>[6x]AEIGGDHGYNATNIAAGQTSGAVTQIGPAVMGMVRRAIPNLIAFDICGVQPMNSPTGQVFALRAVYGKDPVAAGAKEAFHPMYGPDAMFSGQGAAKKFPALAASTQTTVGDIYTHFFQETGTVYLQASVQVTIDAGATDAAKLDAEIKKQMEAGALVEIAEGMATSIAELQEGFNGSTDNPWNEMGFRIDKQVIEAKSRQLKAAYSIELTQDLRAVHGMDADAELSGILATEIMLEINREVVDWINYSAQVGKSGMTLTPGSKAGVFDFQDPIDIRGARWAGESFKALLFQIDKEAVEIARQTGRGEGNFIIASRNVVNVLASVDTGISYAAQGLATGFSTDTTKSVFAGVLGGKYRVYIDQYAKQDYFTVGYKGPNEMDAGIYYAPYVALTPLRGSDPKNFQPVMGFKTRYGIGINPFAESAAQAPASRIQSGMPSILNSLGKNAYFRRVYVKGI;>MTFTVDITPKTPTGVIDETKQFTATPSGQ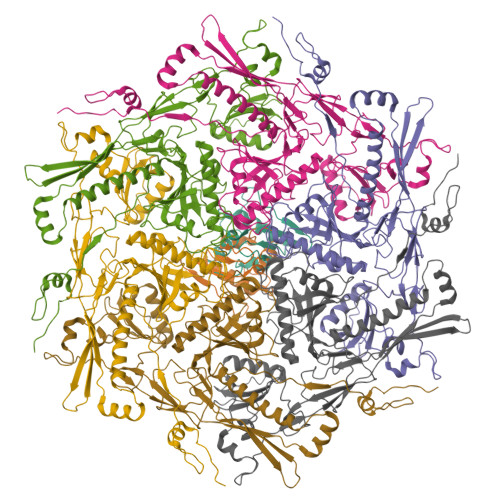TGGGTITYAWSVDNVPQDGAEATFSYVLKGPAGQKTIKVVATNTLSEGGPETAEATTTITVKNKTQTTTLAVTPASPAAGVIGTPVQFTAALASQPDGASATYQWYVDDSQVGGETNSTFSYTPTTSGVKRIKCVAQVTATDYDALSVTSNEVSLTVNKKTMNPQVTLTPPSINVQQDASATFTANVTGAPEEAQITYSWKKDSSPVEGSTNVYTVDTSSVGSQTIEVTATVTAADYNPVTVTKTGNVTVTAKVAPEPEGELPYVHPLPHRSSAYIWCGWWVMDEIQKMTEEGKDWKTDDPDSKYYLHRYTLQKMMKDYPEVDVQESRNGYIIHKTALETGIIYTYP[2x]2-[1-(4-CHLOROBENZOYL)-5-METHOXY-2-METHYL-1H-INDOL-3-YL]-N-[(1R)-1-(HYDROXYMETHYL)PROPYL]ACETAMIDE | C23 H25 Cl N2 O4 | 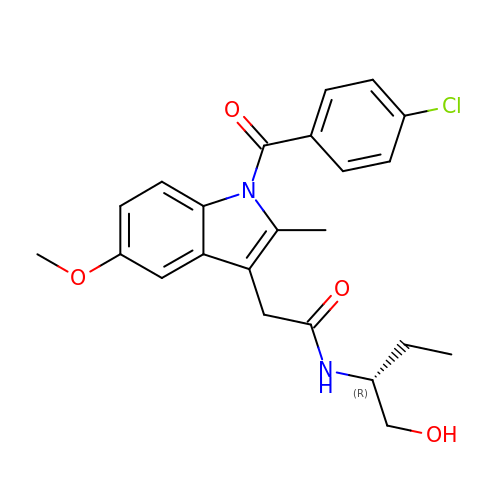GKJWXEORYGBJFS-QGZVFWFLSA-N>[2x]MNHKVHHHHHHIEGRHMTISVPGHGTLGAPDG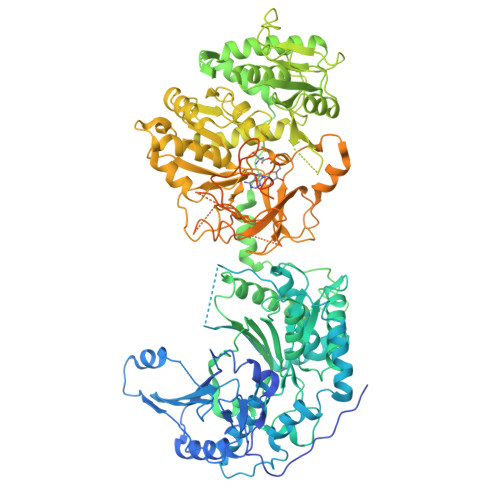AAAPGGEAAELPPLVPEPGDAGQPFPLTPTQQALWVGRADAVDLGDIGCYGYFEWERPELDLARYRRAWERLVAHHPGLRTVVRPDGTQHVLERPGPVPITVEDLRQDPDAVRRLEESRAERGHRALDPGTWPMFDLRVVLLSGRVRVQLGIDLQLMDASSLFLNLFSDLVTLYDDPDAALASQKLAFRDFARWLEEDVRGGARWRADWAYWQERLDGLPPAPDLPAARYGAQGPGKFERCMVRCPAEEFALLRERALAHGLTETELLVGAFAEVLRGWSSDPAFTLNVPVFQRFDVPGIEDVIGDYTNPILLEARPEGRTVAERIVALAARLRADTRHASVNGVEVLRELARRRGLAAAAMPVVVTSLLGLPSAARSITEFGTEVHSITQTPQVSLDFQIRPEDGELRLVWDHRSGAFAPGVVEGAFEAFLDLVGRMLADEPGHGVWEAPFADMRSRRDRAVWNETNDTAEPVPAVLLQERFFAQARRTPDAEAVVASGLRLTYDELARHAYRIGNTLRERGVRPGDLVGVVMEKGWEQYAAVYGILAAGGAYLPIDAASPRGRVARLLESAGAGIVLTQSRLRDELDLPAGTTVLRADTDFETASTAPLTPVQGPDDPAYVIYTSGSTGEPKGVVVAHRGVANLVRDVRRRFAVTPADRLLALSGLHFDASVYDVFGPLACGATVVVPPPFRRAEPDVWAELVRDERVTFWNSVPVLLELLVGEAESRDDRPLATLRLAVVSGDWIPLDLPGRARAQAPGLRVVGSGGPTETICWSLFHPIDAVDPQWTSIPYGKPIANQRYYIVDRDLRPRPTWARGEMAVASPLGLALGYLNDPERTAAKFVTLPGTGERAYLTGDFGRLLPDGGIEILGREDFQVKVAGQRIELGEIEALLHRADGVRAAVVTAPRSSADVVRLQAFVVPETGARLSADALREHLSAELPAAMVPAAIRLLPELPLTANGKVDRLALARLAAAPEEAPEPEARTDYAPRTDVGLLAELVAACVAELLGLDEVPTTGNFFRLGGDALSGTRLASRLQDLLGAPVPIRTVFGNPVLGDLASAIAGDPAAGPQAIRVARLLHTLEEPDEKPGEKPDAEPAGEPDAGSRTSAWSHPQFEK> GLRSTS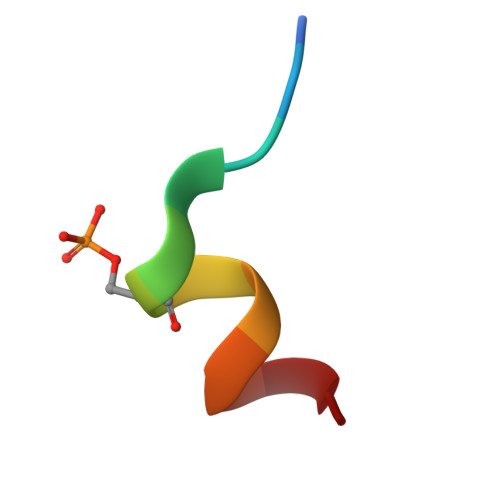YRRAVV>[2x]HNNRLQLSRLERVYQSEQAEKLLLAGVMLRDPARFDLRGTLTHGRDVEIDTNVIIEGNVTLGHRVKIGTGCVIKNSVIGDDCEISPYTV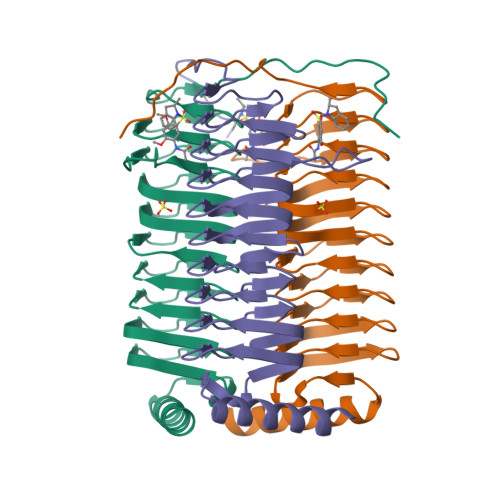VEDANLAAACTIGPFARLRPGAELLEGAHVGNFVEMKKARLGKGSKAGHLTYLGDAEIGDNVNIGAGTITCNYDGANKFKTIIGDDVFVGSDTQLVAPVTVGKGATIAAGTTVTRNVGENALAISRVPQTQKEGWRRPVKKK>MLPNRMALSRQTEDQLKKLKKYTKITPNIAARLAFFRSVESEFRYSPERDSKKLDGTLVLDKITWLGETLQATELVLKMLYPQLEQKALIKAWAAHVE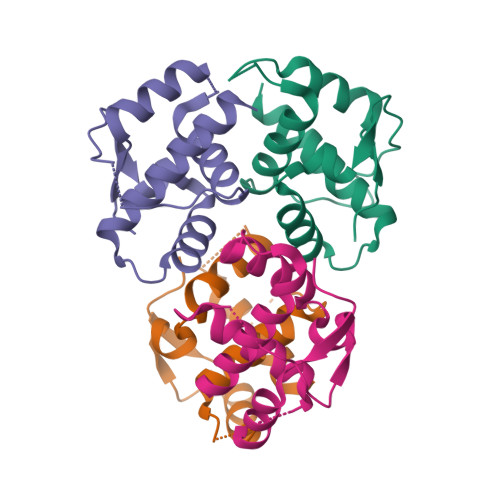DGIAALRNHKSL[4x]> WARGAPRPPPSSPPLSIMGLMPLTKEVAKGSIGRGVLPAVELAIEQIRNESLLRPYFLDLRLYDTECDNAKGLKAFYDAIKYGPNHLMVFGGVCPSVTSIIAESLQGWNLVQLSFAATTPVLADKKKYPYFFRTVPSDNAVNPAILKLLKHYQWKRVGTLTQDVQRFSEVRNDLTGVLYGEDIEISDTESFSNDPCTSVKKLKGNDVRIILGQFDQNMAAKVFCCAYEENMYGSKYQWIIPGWYEPSWWEQVHTEANSSRCLRKNLLAAMEGYIGVDFEPLSSKQIKTISGKTPQQYEREYNNKRSGVGPSKFHGYAYDGIWVIAKTLQRAMETLHASSRHQRIQDFNYTDHTLGRIILNAMNETNFFGVTG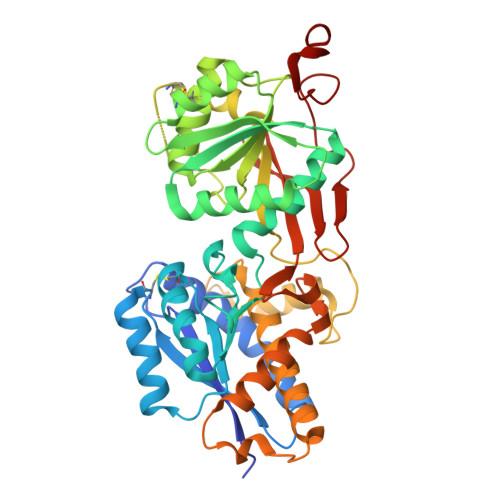QVVFRNGERMGTIKFTQFQDSREVKVGEYNAVADTLEIINDTIRFQGSEPPKDDYKDDDDK>[2x]MAVPSSKEELIKAINSNFSLLNKKLESITPQLAFEPLLEGHAKGTTISVANLVSYLIGWGELVLHWHDQEAKGK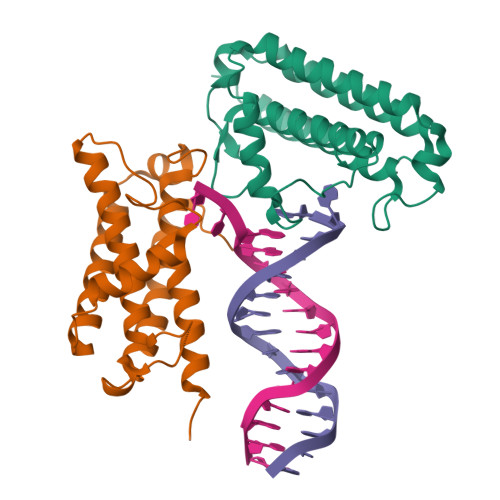TIIFPEEGFKWNELGRLAQKFYRDYEDITEYEVLLARLKENKQQLVALIERFSNDELYGKPWYNKWTRGRMIQFNTASPYKNASGRLNKLQKCLAELEHHHHHH> SLNDDATFWRNARHHLVRYGGTFEPMIIERAKGSFVYDADGRAILDFTSGQMSAVLGHCHPEIVSVIGEYAGKLDHLFSGMLSRPVVDLATRLANITPPGLDRALLLSTGAESNEAAIRMAKLVTGKYEIVGFAQSWHGMTGA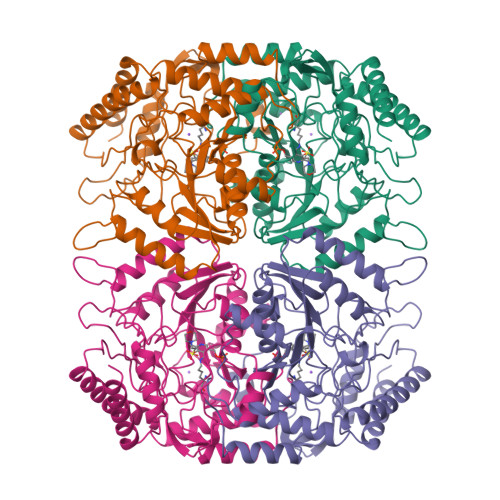AASATYSAGRKGVGPAAVGSFAIPAPFTYRPRFERNGAYDYLAELDYAFDLIDRQSSGNLAAFIAEPILSSGGIIELPDGYMAALKRKCEARGMLLILDEAQTGVGRTGTMFACQRDGVTPDILTLSKTLGAGLPLAAIVTSAAIEERAHELGYLFYTTHVSDPLPAAVGLRVLDVVQRDGLVARANVMGDRLRRGLLDLMERFDCIGDVRGRGLLLGVEIVKDRRTKEPADGLGAKITRECMNLGLSMNIVQLPGMGGVFRIAPPLTVSEDEIDLGLSLLGQAIERAL> MSIAVGMIETRG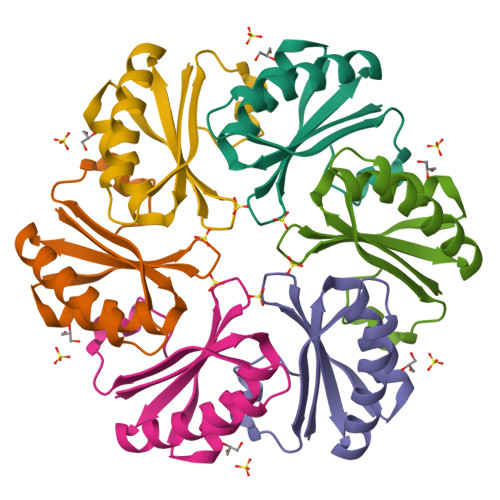FPAVVEAADSMVKAARVTLVGYEKIGSGRVTVIVRGDVSEVQASVSAGIEAANRVNGGEVLSTHIIARPHENLEYVLPILEHHHHHH> MTMKKMFPVLLLGGLLLAGCGTVGLGSGRVNVGVDVGDAGSEQVATL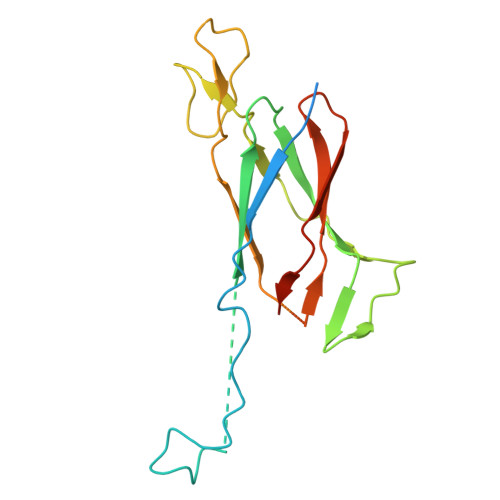TITPEKCDDKGVCTPQKQELSITDGQPVTFTFTARPGSEAVTIEGYRVLSDRLDGVERADPKNPVENAKMNLYVPSGYACEGLTAGASCQGNESDIRIANGQPVQHQIYFASGLGARAAAKGANVTRVVDLEFYGFSANNVPFTRKVTGIVSQGSYVVKTN>[2x]MEETVDPNQKVIALTFDDGPNPATTNQILDSLKKYKGHATFFVLGSRVQYYPETL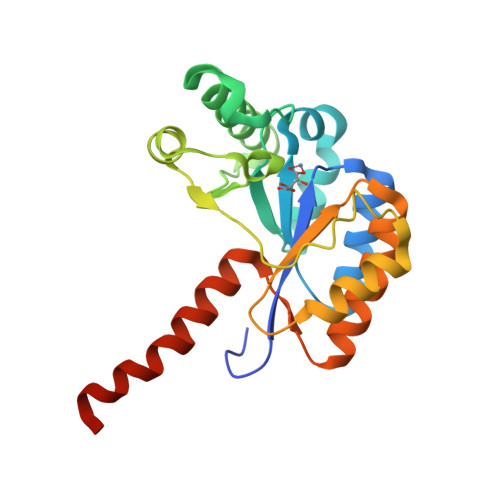IRMLKEGNEVGNHSWSHPLLTRLSVKEALKQINDTQDIIEKISGYRPTLVRPPYGGINDELRSQMKMDVALWDVDPEDWKDRNKKTIVDRVMNQAGDGRTILIHDIYRTSADAADEIIKKLTDQGYQLVTVSQLEEVKKQREAKELRRQWSHPQFEK> MNARSTGQHPARYPGAAAGEPTLDSWQEPPHNRWAFAHLGEMVPSAAVSRRPVNA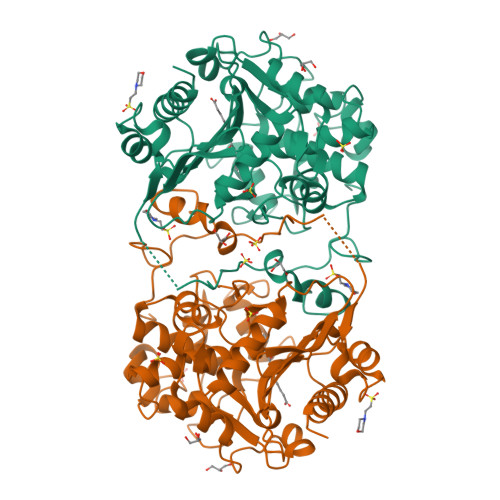PGHALARLGAIAAQLPDLEQRLEQTYTDAFLVLRGTEVVAEYYRAGFAPDDRHLLMAVSKSLCGTVVGALVDEGRIDPAQPVTEYVPELAGSVYDGPSVLQVLDMQISIDYNEDYVDPASEVQTHDRSAGWRTRRHGDPADTYEFLTTLRGDGSTGEFQYCSANTDVLAWIVERVTGLRYVEALSTYLWAKLDADRDATITVDTTGFGFAHGGVSCTARDLARVGRMMLDGGVAPGGRVVSEDWVRRVLAGGSHEAMTDKGFTNTFPDGSYTRQWWCTGNERGNVSGIGIHGQNLWLDPLTDSVIVKLSSWPDPDTEHWHRLQNGILLDVSRALDAV> MTSQIQKWGNSLALRIPKA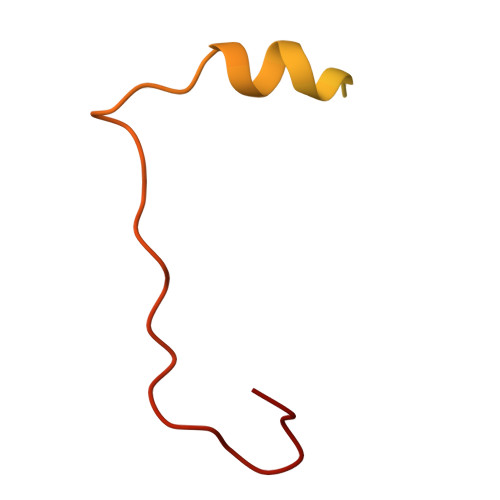LAQQVGLTQSSEVELLLQDGQIVIRPVPARQYDLAALLAEMTPENLHGETDWGALEGREEW>HHHHHHSSGLVPRGSHMQSMRFMILALLVQFLPAWAINDPAKSAAPYHDEFPLFRSANMASPDKLSTGIGFHSFRIPAVVRTTTGRILAFAEGRRHTNQDFGDINLVYKRTKTTANNGASPSDWEPLREVVGSGAGTWGNPTPVVDDDNTIYLFLSWNGATYSQNGKDVLPDGTVTKKIDSTWEGRLHLYLTESRDDGNTWSKPVDLTKELTPDGWAWDAVGPGNGIRLTTGELVIPAMGRNIIGRGAPGNRTWSVQRLSGAGAEGTIVQTPDGKLYRNDRPSQKGYRMVARGTLEGFGAFAPDAGLPDPACQGSVLRYNSDAPARTIFLNSASGTSRRAMRVRISYDADAKKFNYGRKLEDAKVSGAGHEGGYSSMTKTGDYKIGA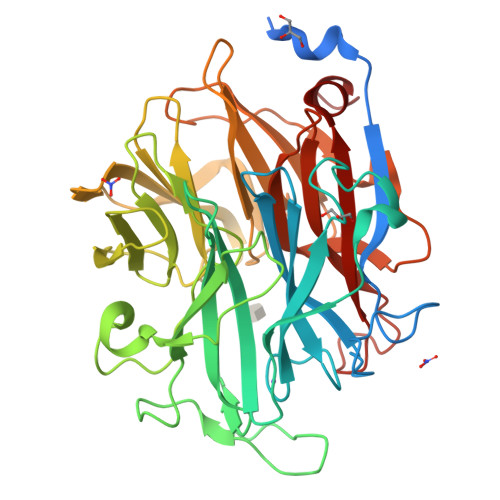LVESDFFNDGTGKNSYRAIIWRRFNLSWILNGPNN[2x]> TLTKHEQDILLKELGPHVDTPAHIVETGLGAYHALFTAHPQYISHFSRLEGHTIENVMQSDGIKHYARTLTEAIVHMLKEISNDAEVKKIAAQYGKDHTSRKVTKDEFMSGEPIFTKYFQNLVADAEGKAAVE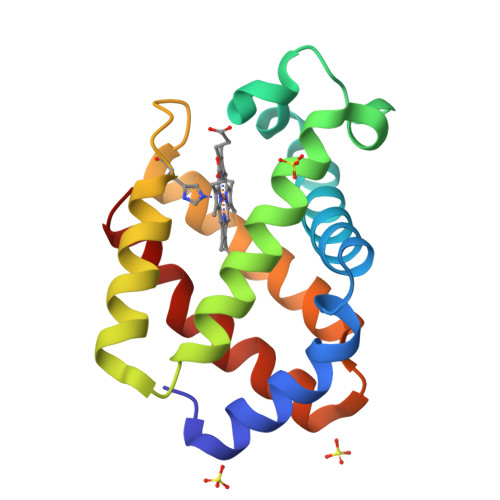KFLKHVFPMMAAEI> MTENIISVDHLTYQYDENQAPALTDVSFTVHAGEWLAIVGHNGSGKSTLAKSLDGLLPFTQGSVTVGGITLTPETVWQVREQIGMIFQNPDNQFVGATVEDDVAFGLENRQISRDEMVPRVQAALAQVGMTSFAQREPSSLSGGQKQRVALAGIVAIAPKILILDEATSMLDPQGRIEMLAIVRQLRQQQNLTVISITHDIDEAASADRVLVIDDGRLVDEAVPSQIFERGTQLVEMGLDLPFTEKLKAALRQRGITPPTTYQTAAEMEEWLWQSLSNT;> MAIAFEHVTYTYQAGTPMAHTALTDVSLTVPDRGYLAIIGHTGSGKSTLIQQLNALLKPTSGTIKIDEFTITPETTNAALKPLRQHVGMVFQFPENQLFEETVRQDIAFGPKNFGMADADALALADEMLTTVGLDQSYAERSPFELSGGQMRRVAIAGVLAMQPKVLVLDEPTAGLDPQGRQEMMRLFARLHQEQGLTIVLVTHQMEDVAQYAEQVAVMHEGRLMKFGTPADVFSNREWLQDHQLDVPQAAQFARRLRDRGLTFPKQPLTADQLADYLAQQWAQRGADHV;> MTKGSLKENTIAAVLIAMTVALSILVVIPIPATKGIVTLCEVGIYTSAILYGRRMGLLVGGASGFLIDILTGYPVWCLFSLVIHGTQGLVVGWLLPRHHKGIRSMLLPLLVGSLVMVIGYCLATTLLFGWPAGLASIFGNVVQVGFGAGVTLSIVGPLTRLKPDLV;> MSNFIFGRYLPLDSVVHRLDPRAKLMLSFCYIIVVFLANNI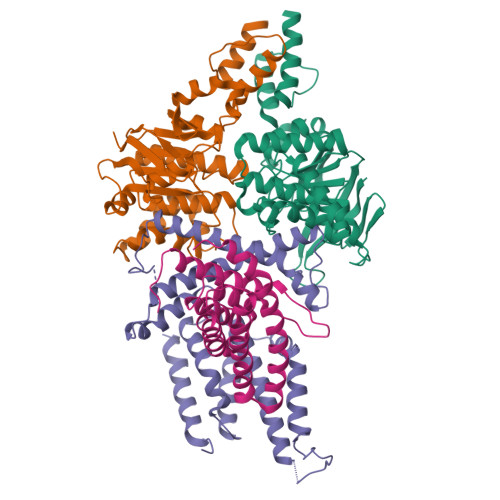WSYAILIAFTVGAILSSKISLGFFLKGIRPLLWLIVFTVVLQLLFSPAGGHTYFHWAFINVTQDGLINAGYIFVRFLLIIMMSTLLTLSTQPLDIATGLASLMKPLRWVKVPVDTLAMMLSIALRFVPTLMDEATKIMNAQRARGVDFGEGGLFKQAKSLIPLMVPLFMSAFNRAEDLSTAMEARGYQDSEHRSQYRILTWQRRDTVTWLLFLLGFVAILIFRHW>[2x]SKIGINGFGRIGRLVLRAALEMGAQVVAVNDPFIALEYMVYMFKYDSTHGMFKGEVKAEDGALVVDGKKITVFNEMKPENIPWSKAGAEYIVESTGVFTTIEKASAHFKGGAKKV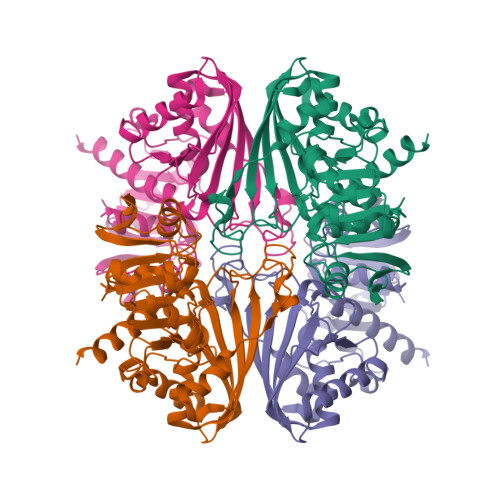IISAPSADAPMFVCGVNLEKYSKDMKVVSNASCTTNCLAPVAKVLHENFEIVEGLMTTVHAVTATQKTVDGPSAKDWRGGRGAAQNIIPSSTGAAKAVGKVIPELDGKLTGMAFRVPTPNVSVVDLTVRLGKECSYDDIKAAMKAASEGPLQGVLGYTEDDVVSCDFTGDNRSSIFDAKAGIQLSKTFVKVVSWYDNEFGYSQRVIDLIKHMQKVDSA>MGKYFGTDGVRGVANSELTPELAFKVGRFGGYVLTKDKQRPKVLIGRDTRISGHMLEGALVAGLLSIGAEVMRLGVISTPGVSYLTKAMDAEAGVMISASHNPVQDNGIKFFGGDGFKLSDEQEAEIERLMDEPEDKLPRPVGADLGLVNDYFEGGQKYLQFLKQTADEDFTGIHVALDCANGATSSLATHLFADLDADVSTMGTSPNGLNINDGVGSTHPEALSAFVKEKNADLGLAFDGDGDRLIAVDEKGNIVDGDQIMYICSKHLKSEGRLKDDTVVSTVMSNLGFYKALEKEGIKSVQTAVGDRYVVEAMKKDGYNVGGEQSGHLIFLDYNTTGDGLLSAIMLMNTLKATGKPLSELAAEMQKFPQLLVNVRVTDKYKVEENEKVKAVISEVEKEMNGDGRILVRPSGTEPLVRVMAEAKTKELCDEYVNRIVEVVRSEMGLELVPRGSSGLEHHHHHH[6x];>EAQQKTIEAITKAINYMAKRRIGALLTIERDTGMGDYIETGIPLNAKVSSELLINIFIPNTPLHDGAVIMKNNEIAAAACYLPLSESPFISKELGTRHRAAVGISEVTDSLTIIVSEETGGVSVAKNGDLHRELTEEALKEMLEAEFKKNTRDTSSNRWYWRGKKNG[6x]

GlmM is a phosphoglucomutase enzyme catalyzing the conversion of glucosamine-6-phosphate to glucosamine-1-phosphate, which is subsequently used to produce the essential peptidoglycan precursor UDP-N-acetyl-glucosamine. CdaA (also referred to as DacA in some bacteria) is a membrane-bound cyclase with three predicted N-terminal transmembrane helices and a cytoplasmic catalytic DAC domain. c-di-AMP is formed from two molecules of ATP by enzymes containing a DAC domain. As part of the current study, we investigated how the activity the B. subtilis c-di-AMP cyclase CdaA is regulated by GlmM, a phosphoglucomutase enzyme required for the synthesis of an essential peptidoglycan precursor.

On the other hand, diffracting crystals were obtained for the CdaACD:GlmMF369 complex, in which the GlmM protein lacks the flexible C-terminal domain 4. The crystals were obtained under two different conditions (see Experimental procedures section), and the structure of the CdaACD:GlmMF369 complex could be solved at 3.6 Å (Complex 1) and at 4.2 Å (Complex 2) by molecular replacement using the B. subtilis CdaACD and GlmM (dimer) structures as search models. Furthermore, in both complex structures, three complex molecules were obtained in the asymmetric unit and each complex was composed of a GlmMF369 dimer and a CdaACD dimer in the inactive dimer configuration. Since the obtained complex structures were basically identical, all further descriptions are based on the higher resolution complex 1 structure. In the complex, a CdaACD dimer was positioned in the large groove at the top of the GlmMF369 dimer and formed interactions with domain 2 of GlmM. The complex was asymmetric, with one of the CdaACD monomers, CdaACD(2) (shown in light blue in Fig. 4) placed in the center of the GlmMF369 groove and the other monomer, CdaACD(1) (shown in dark blue in Fig. 4) projecting toward the solvent. PDBePISA analysis revealed an average buried surface area of 996 Å2 in the interface between GlmMF369(1) and the CdaACD dimer, which was stabilized by four hydrogen bond and four ionic bond interactions between GlmMF369(1) and CdaACD(1) and five hydrogen bond and three ionic bond interactions with CdaACD(2). The main interactions in the complex were formed between three residues, D151, E154, and D194 of domain 2 in GlmMF369(1) and residue R126 in each of the CdaACD monomers. The active site in CdaACD(2) was completely occluded upon interaction with the GlmMF369 dimer (dark blue CdaACD monomer with active site region highlighted in yellow) but the active site in CdaACD(1) appeared at least partially exposed (light blue CdaACD monomer with active site region highlighted in green). Although the active site of the CdaACD(1) was exposed and accessible in the complex with GlmMF369, in an active dimer conformation, parts of the second CdaACD molecule would collide and overlap with GlmMF369, highlighting that also CdaACD(1) cannot form active head-to-head oligomers in the complex.1-(3,4,DIHYDROXY-5-NITROPHENYL)-3-{4-[3-(TRIFLUOROMETHYL) PHENYL] PIPERAZIN-1-YL}PROPAN-1-ONE | C20 H20 F3 N3 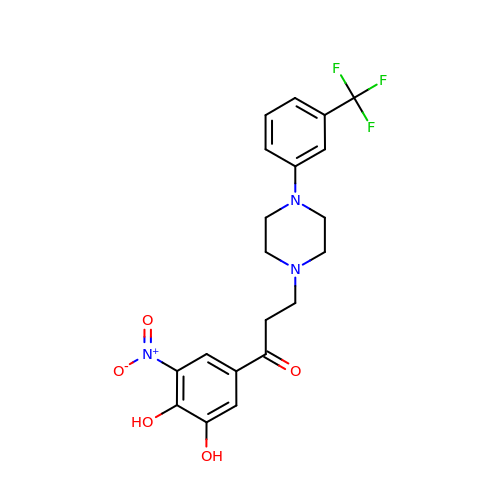O5 | KVIVJQWOYSWCCZ-UHFFFAOYSA-N> MSIVVKNNIHWVGQRDWEVRDFHGTEYKTLRGSSYNSYLIREEKNVLIDTVDHKFSREFVQNLRNEIDLADIDYIVINHAEEDHAGALTELMAQIPDTPIYCTANAIDSINGHHHHPEWNFNVVKTGDTLDIGNGKQLIFVETPMLHWPDSMMTYLTGDAVLFSNDAFGQHYCDEHLFNDEVDQTELFEQCQRYYANILTPFSRLVTPKITEILGFNLPVDMIATSHGVVWRDNPTQIVELYLKWAADYQEDRITIFYDTMSNNTRMMADAIAQGIAE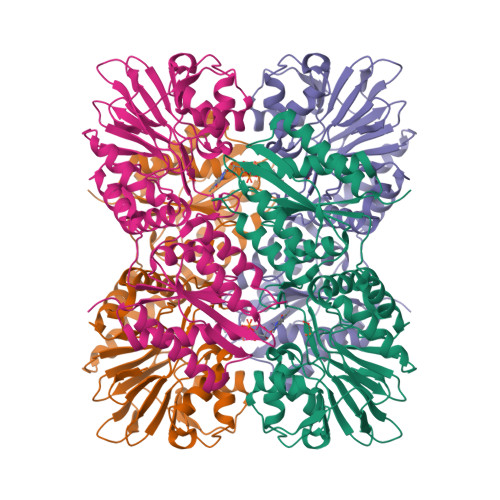TDPRVAVKIFNVARSDKNEILTNVFRSKGVLVGTSTMNNVMMPKIAGLVEEMTGLRFRNKRASAFGSHGWSGGAVDRLSTRLQDAGFEMSLSLKAKWRPDQDALKLCREHGREIARQWALAPLPQSTVNTVVKEETSATTTADLGPRMQCSVCQWIYDPAKGEPMQDVAPGTPWSEVPDNFLCPECSLGKDVFEELASEAK> MKITVLGCGALGQLWLTALC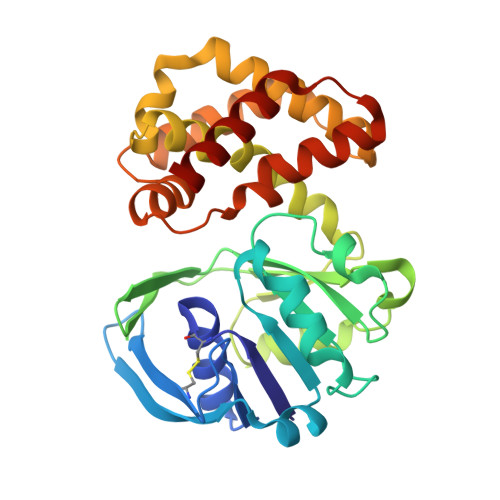KQGHEVQGWLRVPQPYCSVNLVETDGSIFNESLTANDPDFLATSDLLLVTLKAWQVSDAVKSLASTLPVTTPILLIHNGMGTIEELQNIQQPLLMGTTTHAARRDGNVIIHVANGITHIGPARQQDGDYSYLADILQTVLPDVAWHNNIRAELWRKLAVNCVINPLTAIWNCPNGELRHHPQEIMQICEEVAAVIEREGHHTSAEDLRDYVMQVIDATAENISSMLQDIRALRHTEIDYINGFLLRRARAHGIAVPENTRLFEMVKRKESE Aromatic amino acid decarboxylase (AADC) deficiency is a severe inherited recessive neurotransmitter disorder caused by an impairment in dopamine synthesis due to the lack/modification of AADC, the enzyme converting l‐dopa to dopamine. Patients exhibit severe movement disorders and neurodevelopmental delay, with a high risk of premature mortality.

We then transfected the DDC‐KO cells with two AADC catalytic variants, R347Q and L353P, which resulted in loss‐of‐function and an altered profile of dopamine metabolites. By combining several structural approaches (X‐ray crystallography, molecular dynamics, small angle X‐ray scattering, dynamic light scattering, and spectroscopy), we determined that both variants alter the flexibility of the structural element to which they belong, whose integrity is essential for catalysis. This change causes a mispositioning of essential residues at the active site, leading, in turn, to an unproductive external aldimine, identifying the molecular basis for the loss‐of‐function.

> MNASEFRRRGKEMVDYVANYMEGIEGRQVYPDVEPGYLRPLIPAAAPQEPDTFEDIINDVEKIIMPGVTHWHSPYFFAYFPTASSYPAMLADMLCGAIGCIGFSWAASPACTELETVMMDWLGKMLELPKAFLNEKAGEGGGVIQGSASEATLVALLAARTKVIHRLQAASPELTQAAIMEKLVAYSSDQAHSSVERAGLIGGVKLKAIPSDGNFAMRASALQEALERDKAAGLIPFFMVATLGTTTCCSFDNLLEVGPICNKEDIWLHVDAAYAGSAFICPEFRHLLNGVEFADSFNFNPHKWLLVNFDCSAMWVKKRTDLTGAFRLDPTYLKHSHQDSGLITDYQHWQIPLGRRFRSLKMWFVFRMYGVKGLQAYIRKHVQLSHEFESLVRQDPRFEICVEVILGLVCFRLKGSNKVNEALLQRINSAKKIHLVPCHLRDKFVLRFAICSRTVESAHVQRAWEHIKELAADVLRAERE>TPEMPVLENRAAQGDITAPGGARRLTGDQTAALRDSLSDKPAKNIILLIGDGMGDSEITAARNYAEGAGGFFKGIDALPLTGQYTHYALNKKTGKPDYVTDSAASATAWSTGVKTYNGALGVDIHEKDHPTILEMAKAAGLATGNVSTAELQDATPAALVAHVTSRKCYGPSATSEKCPGNALEKGGKGSITEQLLNARADVTLGGGAKTFAETATAGEWQGKTLREQAQARGYQLVSDAASLNSVTEANQQKPLLGLFADGNMPVRWLGPKATYHGNIDKPAVTCTPNPQRNDSVPTLAQMTDKAIELLSKNEKGFFLQVEGASIDKQDHAANPCGQIGETVDLDEAVQRALEFAKKEGNTLVIVTADHA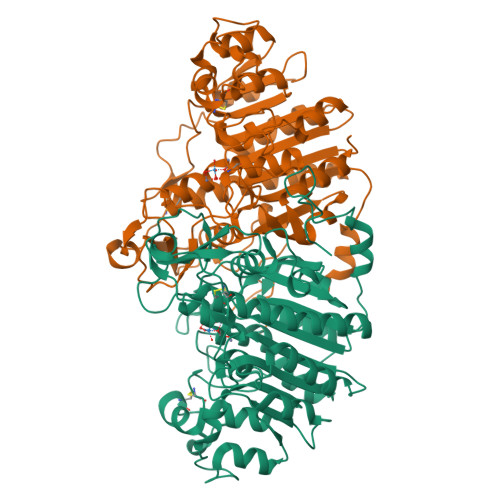HASQIVAPDTKAPGLTQALNTKDGAVMVMSYGNSEEDSQEHTGSQLRIAAYGPHAANVVGLTDQTDLFYTMKAALGLKSAWSHPQFEK[2x]>[2x]AMDPMKIADLMTLLDHHVPFSTAESWDNVGLLIGDEDVEVTGVLTALDCTLEVVNEAIEKGYNTIISHHPLIFKGVTSLKANGYGLIIRKLIQHDINLIAMHTNLDVNPHGVNMMLAKVMGLKNISIINNQQDVYYKVQTYIPKDNVGPFKDKLSENGLAQEGNYEYCFFESEGRGQFKPVGEANPTIGQIDKIEDVDEVKIEFMIDAYQK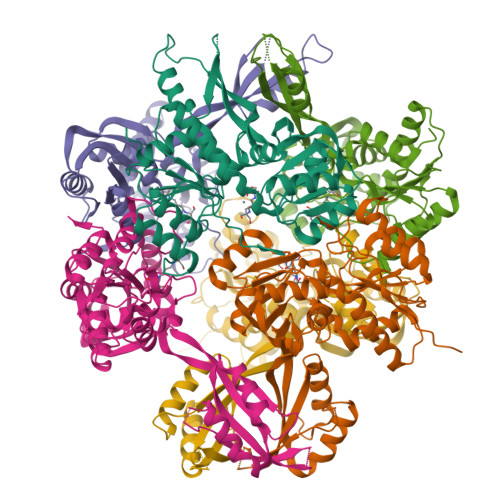SRAEQLIKQYHPYETPVFDFIEIKQTSLYGLGVMAEVDNQMTLEDFAADIKSKLNIPSVRFVGESNQKIKRIAIIGGSGIGYEYQAVQQGADVFVTGDIKHHDALDAKIHGVNLIDINHYSEYVMKEGLKTLLMNWFNIEKINIDVEASTINTDPFQYI>MAYDDLHEGYATYTGSGYSGGAFLLDPIPSDMEITAINPADLNYGGVKAALAGSYLEVEGPKGKTTVYVTDLYPEGARGALDLSPNAFRKIGNMKDGKINIKWRVVKAPITGNFTYRIKEGSSRWWAAIQVRNH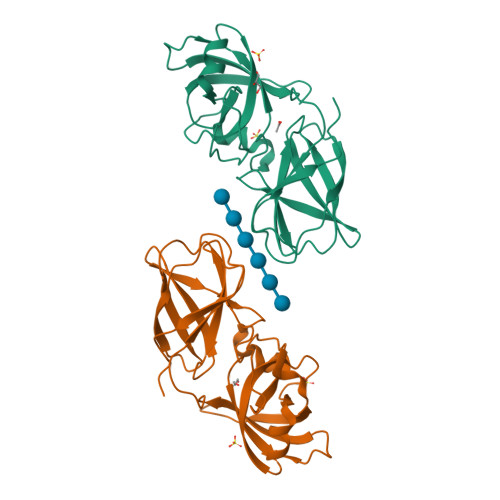KYPVMKMEYEKDGKWINMEKMDYNHFVSTNLGTGSLKVRMTDIRGKVVKDTIPKLPESGTSKAYTVPGHVQFPE[2x]6-ethyl-5-{(3S)-3-[3-methoxy-5-(pyridin-4-yl)phenyl]but-1-yn-1-yl}pyrimidine-2,4-diamine | C22 H23 N5 O 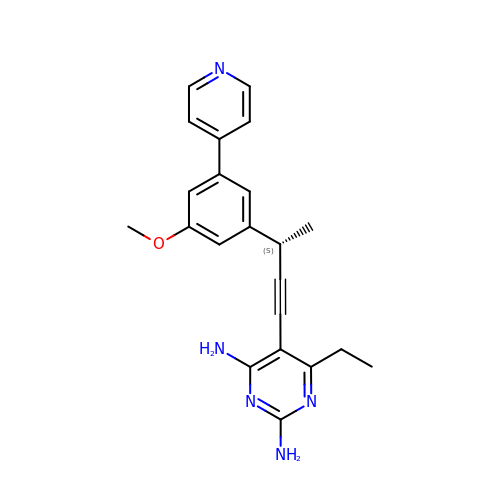| KEPLBUUTAQCZOE-CQSZACIVSA-N3-chloro-4,6-dihydroxy-5-[(2E,6E,8S)-8-hydroxy-3,7-dimethylnona-2,6-dien-1-yl]-2-methylbenzaldehyde | C19 H25 Cl O4 | 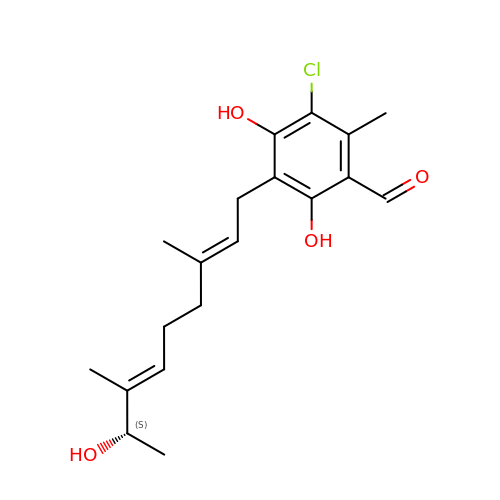OFCDDOBCQZHXDK-KCURMNHOSA-N>MHHHHHHTSKIEQPRWASKDSAAGAASTPDEKIVLEFMDALTSNDAAKLIEYFAEDTMFQAMPLPPAYGRDAVEQTLAGLFTVMSIDAVETFHIGSSNGLVYTERVDVLRALPTGKSYNLSILGVFQLTEGKITGWRDYFDLREFE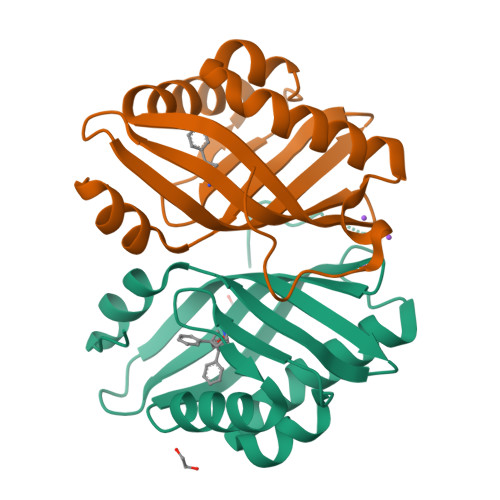EAVDLPLRG[2x]Human serine racemase (hSR) catalyses racemisation of L-serine to D-serine, the latter of which is a co-agonist of the NMDA subtype of glutamate receptors that are important in synaptic plasticity, learning and memory. In mammals, D-serine is synthesised by a pyridoxal-5′-phosphate (PLP)-containing enzyme serine racemase (SR). The first mammalian structures of SR, published in 201031, revealed a dimeric structure with each subunit consisting of a small domain (residues 78–153) and a large domain (residues 4–67 and 156–316). The roles of Ser 84 and Lys 56 as the Si and Re-face acid/bases in the catalytic cycle of hSR are generally accepted.

Analysis of 600 fragment-soaked hSR crystals revealed 44 interesting binding events, of which twelve had displaced Tyr 121 from the core of the small domain in at least one of the four subunits in the asymmetric unit. One of these is a 1.53 Å crystal structure of hSR bound to compound 1-x0495 (Fig. 3a, A-subunit; Supplementary Table 4 for XChem ligand structures). In the hSR XChem structure bound to compound 1-x0495, the compound is observed in subunits A, B and D, but not in the subunit C. A superposition of the 1-x0495 structure with the 1.6 Å malonate/ATP structure shows the Tyr 121 sidechains occupying similar positions in both structures. However, the structure with 1-x0495 bound remains in the ‘open’ conformation, with a cleft between the small and large domain that is accessible to substrate, whereas the structure with malonate and ATP is in the ‘closed’ conformation with Ser 84 in proximity to the malonate. The twelve XChem compounds binding to the Tyr 121 region exploit a naturally occurring pocket. Before the small domain can move to enclose the substrate (or malonate), Tyr 121 needs to be expelled from the core of the small domain so that it can adopt the ‘closed’ catalytic hSR conformation.

>MDAQYDISFADVEKAHINIRDSIHLTPVLTSSILNQLTGRNLFFKCELFQKTGSFKIRGALNAVRSLVPDALERKPKAVVTHSSGNHGQALTYAAKLEGIPAYIVVPQTAPDCKKLAIQAYGASIVYCEPSDESRENVAKRVTEETEGIMVHPNQEPAVIAGQGTIALEVLNQVPLVDALVVPVGGGGMLAGIAITVKALKPSVKVYAAEPSNADDCYQSKLKGKLMPNLYPPETIADGVKSSIGLNTWPIIRDLVDDIFTVTEDEIKCATQLVWERMKLLIEPTAGVGVAAVLSQHFQTVSPEVKNICIVLSGGNVDLTSSITWVKQAERPASYQSVSVHHHHHH[4x]> MIKAKTYPDFKEFVKDFVANVKAGKRYDFRKYQEAVLPLTYSSPWPESD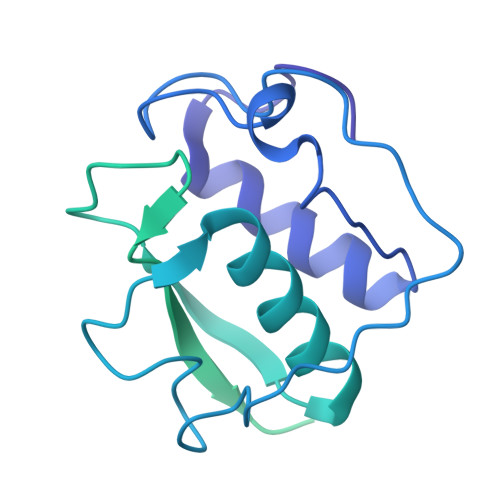IPEVTDFNYTPDYTVPFSEELLYSVGAQMRTADFFMDLQYAIINGKDVDTVYCEWLARVKPFSMLNAKLKDSAQPPVITTQPTGGAVNEGSAINLSIVATNATSYQWKKGSSDISGATSATYTKAGAVPADAGSYTCVVTNDVGSTTSDAAVITINPLPVITTQPTSKAVNESSTLTLSVVATGATSYQWKKNGTNISGATSATYSKANAKTTDAGSYTCVVTNAVGSVTSNAATVTINPLPVITVQPQDQDLTVGQTLTISITATGATGYQWRKGNSNISGATSATYTKASVTTADDGNYDCVVTNAVGSVTSHQAKVQVTA Guaiacol 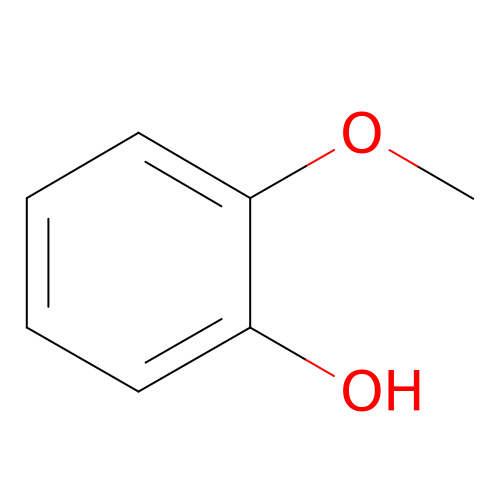| C7 H8 O2 | LHGVFZTZFXWLCP-UHFFFAOYSA-N BEST1-4 proteins are expressed in the plasma membrane and form Ca2+-activated Cl- channels by assembling as pentamers. The channel comprises five BEST1 subunits arranged symmetrically around a central ion pore that is ~95 Å long. The diameter of the pore varies along its length and contains two constrictions, the ‘neck’ and the ‘aperture’, both of which are lined by hydrophobic amino acids. To address these questions we determined a series of cryo-electron microscopy (cryo-EM) structures of chicken BEST1 with and without Ca2+ in activated, deactivated, and inactivated states that represent the major gating transitions of the channel.

The structure is determined to 3.0 Å resolution and is indistinguishable from a cryo-EM structure of Ca2+-free BEST1405 at 3.6 Å resolution. The neck is closed in the absence of Ca2+, and notably, it shares the same closed conformation as in the inactivated and Ca2+-bound closed structures. The overall structure of the channel is very similar to the inactivated and Ca2+-bound closed conformations with the only notable differences near the Ca2+ clasp. In structures with Ca2+ bound, the five Ca2+ clasps, one from each subunit, resemble a belt that wraps around the midsection of BEST1. Without Ca2+, the majority of each Ca2+ clasp becomes disordered. 3D classification of the Ca2+-free BEST1345 dataset yielded only closed conformations of the neck but did indicate a degree of flexibility in the channel between the transmembrane and cytosolic regions that was manifested as a ~ 5° rotation along the symmetry axis. This conformational flexibility was not observed in the Ca2+-bound datasets, which suggests that Ca2+ binding rigidifies the channel. We hypothesize that this Ca2+-dependent rigidification may be necessary for opening of the neck. When unoccupied by Ca2+, the Ca2+ clasps are disordered, the neck is closed, and ions are prevented from permeating through the channel by the neck.

>TVTYTNRVADARLGTFSQLLLQWKGSIYKLLYSEFLIFISLYFAISLVYRLILSESQRLMFEKLALYCNSYAELIPVSFVLGFYVSLVVSRWWAQYESIPWPDRIMNLVSCNVDGEDEYGRLLRRTLMRYSNLCSVLILRSVSTAVYKRFPSMEHVVRAGLMTPEEHKKFESLNSPHNKFWIPCVWFSNLAVKARNEGRIRDSVLLQGILNELNTLRSQCGRLYGYDWISIPLVYTQVVTVAVYSFFLACLIGRQFLDPEKAYPGHELDLFVPVFTFLQFFFYAGWLKVAEQLINPFGEDDDDFETNWLIDRNLQVSLMAVDEMHQDLPILEKDLYWNEPDPQEGEEF[5x]> MRLSYEALEWRTPIENSTEPVSLPPPPPFFGQERAREALELAIRGGFHAYLVGPPSLGKHEALLAYLSTQSVETPPDLLYVPLSERKVAVMTLPSGQEIHLAEAVEGLLLEVNRLDELFRQGSFLREKTQLEARFKEAREQQLEALRREAQEAGFALSTNGERLELTGPGPVPAELSARLEEVTLGSMAASAELEVALRRLRRDWALHYLNNRFEPLFQRFPQARAYLEALRARLARYAETGEPLDPAQWRPNLLTSSSSGTPPPIVYEPYATAPRLFGRLDYLVDRGVWSTNVSLIRP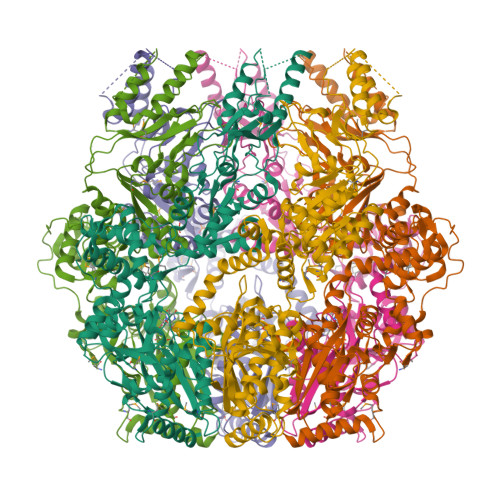GAVHRAQGGYLILDALSLKREGTWEAFKRALRNGQVEPVTEPQAPAGLEVEPFPIQMQVMLVGTPEAFEGLEEDPAFSELFRIRAEFSPTMPASPENCTALGGWLLAQGFQLTQGGLTRLYDEARRMAEQRDRMDARLVEIRALAEEAAVLGGGLLTAESVEQAIAAREHRSFLSEEEFLRAVQEGVIRLRTTGRAVGEVNSLVVVEAAPYWGRPARLTARAAPGRDHLISIDREAGLGGQIFHKAVLTLAGYLRSRMIEHGSLPVTISLAFEQNYVSIEGDSAGLAELVAALSAIGNLPLRQDLAVTGAVDQTGKVLAVGAINAKVEGFFRVCKALGLSGTQGVILPEANLANLTLRAEVLEAVRAGQFHIYAVETAEQALEILAGARMEGFRGLQEKIRAGLEAFARLEEGHDKEDREKLAAALEHHHHHH>MFPEQQKEEFVSVWVRDPRIQKEDFWHSYIDYEICIHTNSMCFTMKTSCVRRRYREFVWLRQRLQSNALLVQLPELPSKNLFFNMNNRQHVDQRRQGLEDFLRKVLQNALLLSDSSLHLFLQSHLNSEDI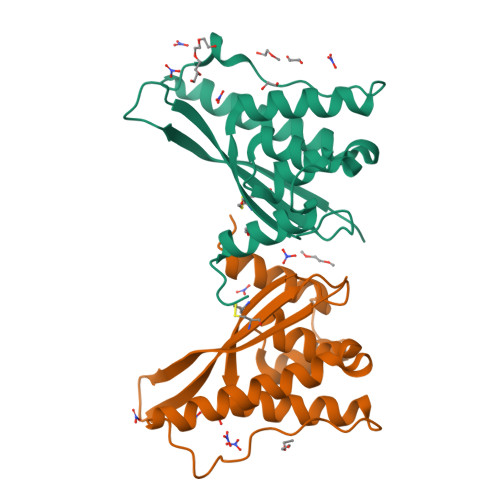EACVSGQTKYSVEEAIHKFALMNRRFPEEDEEGKKENDIDYDSESSSSGLGHSSDDSSSHGCKVNTAPQESLEHHHHHH[2x]The nitrogenase Fe protein mediates ATP-dependent electron transfer to the nitrogenase MoFe protein during nitrogen fixation, in addition to catalyzing MoFe protein-independent substrate (CO2) reduction and facilitating MoFe protein metallocluster biosynthesis. The Fe protein also catalyzes MoFe protein-independent CO2-to-CO reduction, and participates in the biosynthesis of both the P-cluster and FeMo-cofactor. Unlike most Fe4S4 clusters in metalloproteins which adopt two oxidation states, the Fe protein cluster can span three oxidation states (2+/1+/0). The origins of these unusual properties of the Fe protein cluster are not well understood, but may reflect the solvent accessibility of the cluster and its positioning at the dimer interface.

We initially observed Se-incorporation into the Fe protein cluster using our group’s previously reported KSeCN turnover conditions, which include KSeCN as the selenium source, dithionite as the reductant, and an ATP regenerating system. Crystallization of the nitrogenase proteins from the concentrated reaction mixture was achieved by selecting conditions that favor either MoFe protein or Fe protein crystals. The crystal structure at 1.51 Å resolution of the Se-incorporated Fe protein isolated from this reaction mixture is shown in Figure 2. The crystal form is isomorphous to the previously reported MgADP-bound state of the Fe protein, with the Fe protein molecular twofold axis coincident with a crystallographic twofold axis so that the asymmetric unit contains one subunit and half the cluster. The unique Fe1 and Fe2 sites are coordinated to Cys 97A and Cys 132A, respectively, while the unique chalcogenide sites 3 and 4 are buried and surface exposed, respectively. The locations of the Se ions within the protein structure were identified by collecting two sets of anomalous diffraction data: one above (12,668 eV) and one below (12,643 eV) the Se K-edge. Modeling the cluster exclusively as either the Fe4S4 or Fe4Se4 form resulted in substantial positive or negative difference density in the corresponding Fobs − Fcalc difference Fourier maps, respectively. By fixing the chalcogenide B-factor values to a value similar to that of the Fe ions, satisfactory mixed cluster models were obtained (see Methods for refinement details). The Se occupancies at the X3 and X4 positions are shown in Table 1, entry 1, with the buried X3 position exhibiting a greater extent of Se-incorporation relative to the surface exposed X4 position. Based on the crystallographic data, we anticipate that the Se-labeled Fe protein exists in a mixture of Se-containing cluster states (i.e., Fe4S4, Fe4S3Se, Fe4S2Se2, Fe4SSe3, and Fe4Se4 may all be present).

> MAMRQCAIYGKGGIGKSTTTQNLVAALAEMGKKVMIVGCDPKADSTRLILHSKAQNTIMEMAAEAGTVEDLELEDVLKAGYGGVKCVESGGPEPGVGCAGRGVITAINFLEEEGAYEDDLDFVFYDVLGDVVCGGFAMPIRENKAQEIYIVCSGEMMAMYAANNISKGIVKYANSGSVRLGGLICNSRNTDREDELIIALANKLGTQMIHFVPRDNVVQRAEIRRMTVIEYDPKAKQADEYRALARKVVDNKLLVIPNPITMDELEELLMEFGIMEVEDESIVGKTAEEV3-hydroxynaphthalene-2-carboxylic acid | C11 H8 O3 | 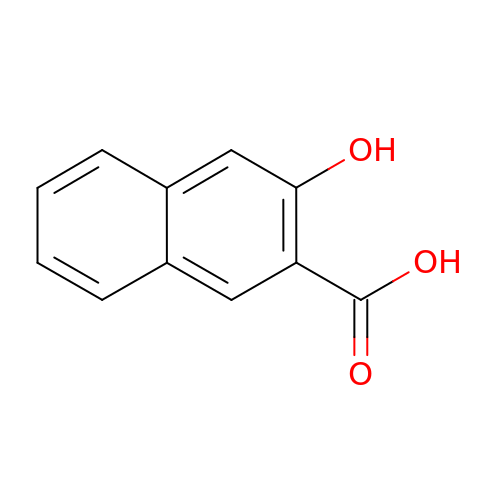ALKYHXVLJMQRLQ-UHFFFAOYSA-N> MENIQKLIARYPLVEDLVALKETTWFNPGATSLAQGLPYVGLTEQDVNAAHDRLARFA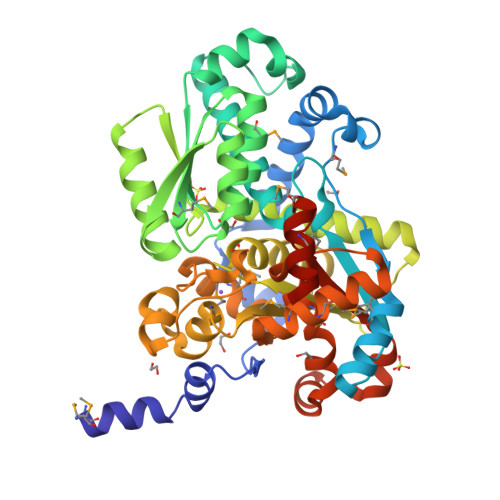PYLAKAFPQTAAAGGMIESDVVAIPAMQKRLEKEYGQTINGEMLLKKDSHLAISGSIKARGGIYEVLTHAEKLALEAGLLTTDDDYSVLLSPEFKQFFSQYSIAVGSTGNLGLSIGIMSACIGFKVTVHMSADARAWKKAKLRSHGVTVVEYEDDYGVAVEQGRKAAQSDPNCFFIDDENSRTLFLGYAVAGQRLKAQFAQQGRVVDASHPLFVYLPCGVGGGPGGVAFGLKLAFGDNVHCFFAEPTHSPCMLLGVYTGLHDAISVQDIGIDNLTAADGLAVGRASGFVGRAMERLLDGLYTLDDQTMYDMLGWLAQEEGIRLEPSALAGMAGPQRICASVAYQQRHGFSQTQLGNATHLVWATGGGMVPEDEMEQYLAKGRLEHHHHHH> GC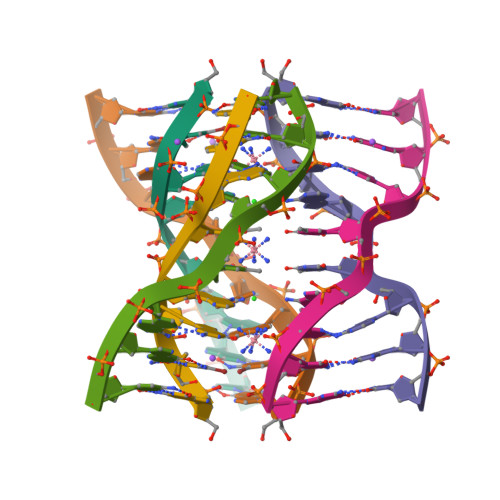GATAGC N-[(2S,3S,4R,5R,6R)-4,5-dihydroxy-2,6-bis(hydroxymethyl)piperidin-3-yl]acetamide | C9 H18 N2 O5 | 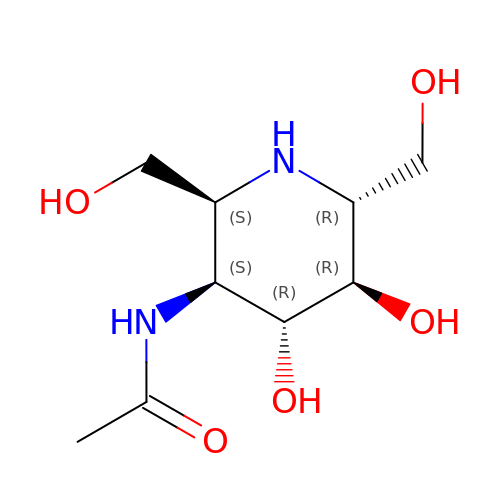GYKHMAHAJKZLAT-SYHAXYEDSA-N> MPFVNKQFNYKDPVNGVDIAYIKIPNVGVMQPVKAFKIHNKIWVIPERDTFTNPEEGDLNPPPEAKQVPVSYYDSTYLSTDNEKDNYLKGVTKLFERIYSTDLGRMLLTSIVRGIPFWGGSTIDTELKVIDTNCINVIQPDGSYRSEELNLVIIGPSADIIQFECKSFGHEVLNLTRNGYGSTQYIRFSPDFTFGFEESLEVDTNPLLGAGKFATDPAVTLAHELIHAGHRLYGIAINPNRVFKVNTNAYYEMSGLEVSFEELRTFGGHDAKFIDSLQENEFRLYYYNKFKDIASTLNKAKSIVGTTASLQYMKNVFKEKYLLSEDTSGKFSVDKLKFDKLYKMLTEIYTEDNFVKFFKVL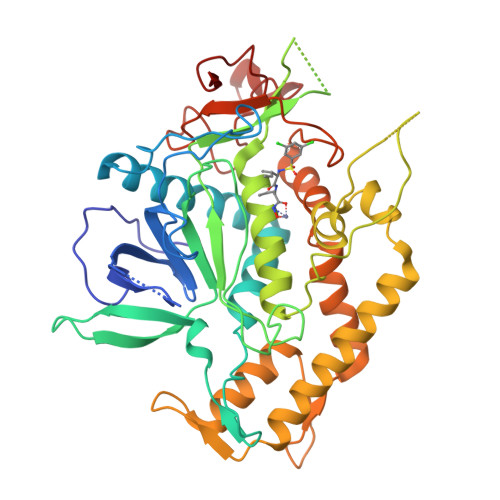NRKTYLNFDKAVFKINIVPKVNYTIYDGFNLRNTNLAANFNGQNTEINNMNFTKLK> MGSSHHHHHHSQGSMHYLDNLLLNTDSYKASHWLQYPPGTDASFFYVESRGGVYDQTAFFGLQSILKEAINRPVTHADIDDAKALLAAHGEPFNEAGWRDIVDRLGGQLPIRIRAVPEGCVVPTHNVLMTIESTDAKAFWVPSYLETLLLRVWYPVTVATVSWQVKQIVRDFLQRTSDDPEGQLPFKLHDFGARGVSSLGSAALGGAAHLVNFLGTDTLSALLLARAHYHTPVAGYSIPAAEHSTITSWGREREVDAYRNMLTQFARPGAIVAVVSDSYDIYRAIREHWGTTLREEIIASGATVVIRPDSGDPVDVVEQCLLLLDEAFGHQVNGKGYKVLNHVRVIQGDGINPQSLRAILERITAAGYAADNVAFGMGGALLQKVDRDTQKFALKCSAVRVDGAWIDVYKDPITDQGKQSKRGRLTLLRDRATGQYRSALLDEVATHAGDSDDALVTVWENGQMLREWTLEQVRAHAD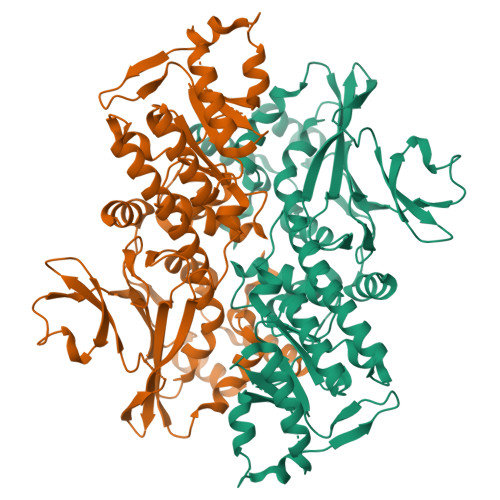AARL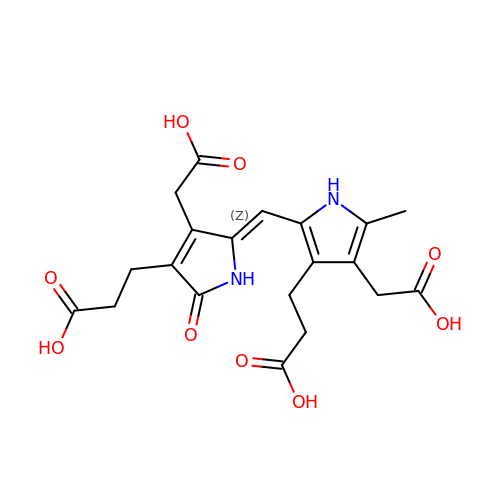3-[(5Z)-5-{[3-(2-carboxyethyl)-4-(carboxymethyl)-5-methyl-1H-pyrrol-2-yl]methylidene}-4-(carboxymethyl)-2-oxo-2,5-dihydro-1H-pyrrol-3-yl]propanoic acid | C20 H22 N2 O9 | MBSNQHZDABRTAT-NVNXTCNLSA-N>GAMGSEPRPTAPSSGAPGLAGVGETPSAAALAAARVELPGTAVPSVPEDAAPASRDGGGVRDEGPAAAGDGLGRPLGPTPSQSRFQVDLVSENAGRAAAAAAAAAAAAAAAGAGAGAKQTPADGEASGESEPAKGSEEAKGRFRVNFVDPAASSSAEDSLSDAAGVGVDGPNVSFQNGGDTVLSEGSSLHSGGGGGSGHHQHYYYDTHTNTYYLRTFGHNTMDAVPRIDHYRHTAAQLGEKLLRPSLAELHDELEKEPFEDGFANGEESTPTRDAVVTYTAESKGVVKFGWINGVLVRCMLNIWGVMLFIRLSWIVGQAGIGLSVLVIMMATVVTTITGLSTSAIATNGFVRGGGAYYLISRSLGPEFGGAIGLIFAFANAVAVAMYVVGFAETVVELLKEHSILMIDEINDIRIIGAITVVILLGISVAGMEWEAKAQIVLLVILLLAIGDFVIGTFIPLESKKPKGFFGYKSEIFNENFGPDFREEETFFSVFEIFFPAATGILAGANISGDLADPQSALPKGTLLAILITTLVYVGIAVSVGSCVVRDATGNVNDTIVTELTNCTSAACKLNFDFSSCESSPCSYGLMNNFQVMSMVSGFTPLISAGIFSATLSSALASLVSAPKIFQALCKDNIYPAFQMFAKGYGKNNEPLRGYILTFLIALGFILIAECNVIAPIISNFFLASYALINFSVFHASLAKSPGWRPAFKYYNMWISLLGAILCCIVMFVINWWAALLTYVIVLGLYIYVTYKKPDVNWGSSTQALTYLNALQHSIRLSGVEDHVKNFRPQCLVMTGAPNSRPALLHLVHDFTKNVGLMICGHVHMGPRRQAMKEMSIDQAKYQRWLIKNKMKAFYAPVHADDLREGAQYLMQAAGLGRMKPNTLVLGFKKDWLQADMRDVDMYINLFHDAFDIQYGVVVIRLKEGLDISHLQGQEELLSSQEKSPGTKDVVVS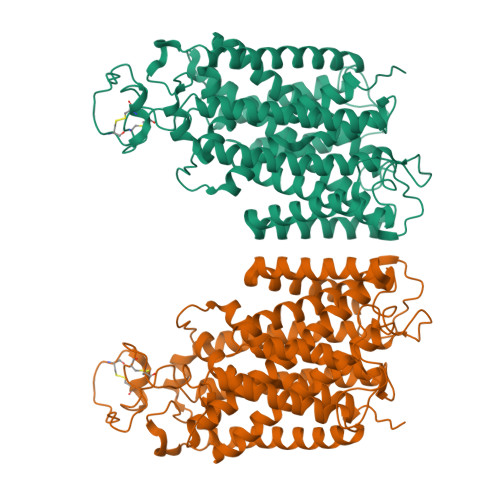VEYSKKSDLDTSKPLSEKPITHKVEEEDGKTATQPLLKKESKGPIVPLNVADQKLLEASTQFQKKQGKNTIDVWWLFDDGGLTLLIPYLLTTKKKWKDCKIRVFIGGKINRIDHDRRAMATLLSKFRIDFSDIMVLGDINTKPKKENIIAFEEIIEPYRLHEDDKEQDIADKMKEDEPWRITDNELELYKTKTYRQIRLNELLKEHSSTANIIVMSLPVARKGAVSSALYMAWLEALSKDLPPILLVRGNHQSVLTFYS[2x]> MLSSLNVLQSSFRGKTALSNSTLLQRPSFAGKEYSLEPIDERTPILFQWFEARPERYEKGEVPILNTKEHPYLSNIINAAKIENERIIGVLVDGNFTYEQKKEFLNLENEHQNIAIIYRADVDFSMYDKKLSDIYLENIHKQESYPASERDNYLLGLLREELKNIPEGKDSLIESYAE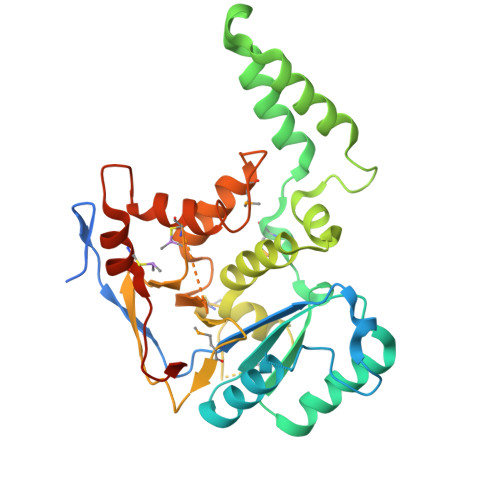KREHTWFDFFRNLAILKAGSLFTETGKTGCHNISPCSGCIYLDADMIITDKLGVLYAPDGIAVHVDCNDEIKSLCNGAIVVNRSNHPALLAGLDIMKSKVDAHPYYDGLGKGIKRHFNYSSLHNYNAFCDFIEEGNPGIIIPNTSMYTSSSW>KVQHIQLLQKNVRAQLVDMKR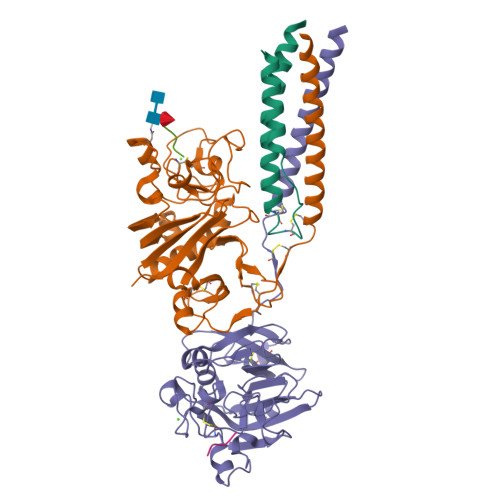LEVDIDIKIRSCRGSCSRALAREVDLKDYEDQQKQLEQVIA[2x];>IPTNLRVLRSILENLRSKIQKLESDVSAQMEYCRTPCTVSCNIPVVSGKECEEIIRKGGETSEMYLIQPDSSVKPYRVYCDMNTENGGWTVIQNRQDGSVDFGRKWDPYKQGFGNVATNTDGKNYCGLPGEYWLGNDKISQLTRMGPTELLIEMEDWKGDKVKAHYGGFTVQNEANKYQISVNKYRGTAGNALMDGASQLMGENRTMTIHNGMFFSTYDRDNDGWLTSDPRKQCSKEDGGGWWYNRCHAANPNGRYYWGGQYTWDMAKHGTDDGVVWMNWKGSWYSMRKMSMKIRPFF[2x];>[2x]THDSSIRYLQEIYNSNNQKIVNLKEKVAQLEAQCQEPCKDTVQIHDITGKDCQDIANKGAKQSGLYFIKPLKANQQFLVYCEIDGSGNGWTVFQKRLDGSVDFKKNWIQYKEGFGHLSPTGTTEFWLGNEKIHLISTQSAIPYALRVELEDWNGRTSTADYAMFKVGPEADKYRLTYAYFAGGDAGDAFDGFDFGDDPSDKFFTSHNGMQFSTWDNDNDKFEGNCAEQDGSGWWMNKCHAGHLNGVYYQGGTYSKASTPNGYANGIIWATWKTRWYSMKKTTMKIIPFNRLTI;>GPRP[4x]> MPEICPRCGLPKELCVCEEIAKEEQKIKIYVTK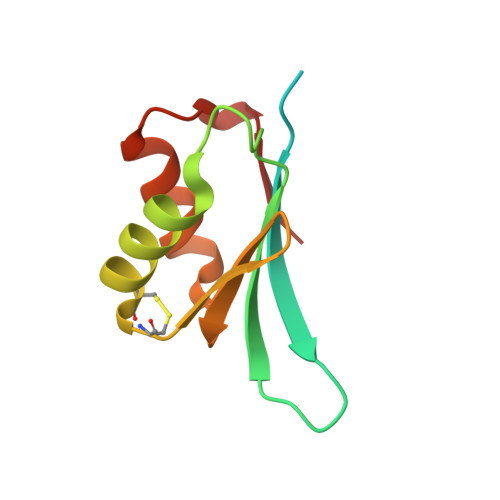RRFGKLMTIIEGFDTSVIDLKELAKKLKDICACGGTVKDNTIELQGDHRKKVAEELVKMGFSRDSIEIR>GPLGSPEFDNNIENIGDGAEVVKRTEDTSSDKWGVTQNIQFDFVKDKKYNKDALILKMQGFINSKTTYYNYKNTDHIKAMRWPFQYNIGLKTNDPNVDLINYLPKNKIDSVNVSQTLGYNIGGNFNSGPSTGGNGSFNYSKTISYNQQNYISEVEHQNSKSVQWGIKANSFITSLGKMSGHDPNLFVGYKPYSQNPRDYFVPDNELPPLVHSGFNPSFIATVSHEKGSGDTSEFEITYGRNMDVTHATRRTTHYGASYLEGSRIHNAFVNRNYTVKYEVNWKTHEIKVKGHN[4x]

With the exception of α-hemolysin, which is homo-heptameric, leukotoxins are bipartite toxins, formed by the non-covalent association of two distinct proteins, a class S and a class F component of approximately 31 and 34 kDa, respectively, into a likely octameric species. Panton-Valentine leukocidin (PVL) is associated with necrotizing skin infections, such as boils, and plays an important role in the poor prognosis of necrotizing pneumonia. Two additional structural domains are also found: the rim domain anchors the protein to the membrane surface, while the stem domain, closely apposed to the core β-sandwich in the soluble form, contributes two β-strands to the pore β-barrel. Since the binding of LukS-PV to the membrane is a saturable process, the necessary presence of a LukS-PV receptor on the cell surface was thus proposed. This was recently confirmed by Spaan et al. who showed that the C5a receptor is required for the binding of LukS-PV to human neutrophils.

Five mutants (Y181A, K182A, H245A, Y246A and N248A) were partially affected. LukS-PV mutants Y181A, K182A, Y246A and N248A also had a significantly decreased calcium entry slope, from 65% to 75% of the control (p<0.05, one-way ANOVA). The T244A, Y246A and N248A mutated proteins crystallized in identical conditions (50% PEG 200, 0.1 M MES-NaOH, pH 7.50). The corresponding crystals belonged to the P43212 space group, with similar cell parameters (a = b∼94 Å and c∼308 Å) and 4 molecules per asymmetric unit. These crystals diffracted X-rays at medium resolution (2.50 to 2.80 Å). In the case of the rim domain, wild-type LukS-PV and mutants T244A, Y246A and N248A displayed only small differences, with r.m.s. deviations comprised between 0.20 Å and 0.30 Å, whereas the structure of the rim domain of the Y184A and Y250A mutants were markedly different, with r.m.s. deviations of 1.10 Å and 1.28 Å, respectively, when compared to the wild-type LukS-PV structure. Residues R73, H245, Y246 and N248 are specific to the two proteins, whereas Y184 of LukS-PV is replaced by a histidine residue in HlgC.>GVIKPDMKIKLKMEGNVNGHAFVIEGEGEGKPYDGTNTINLEVKEGAPLPFSYDILTNAFAYGNRAFTKYPDDIPNYFKQSFPEGYSWERTMTFEDKGIVKVKSDISMEEDSFIYEIHLKGENFPPNGPVMQKKTLKWEPSTEILYVRDGVLVGDIKHKLLLEGGG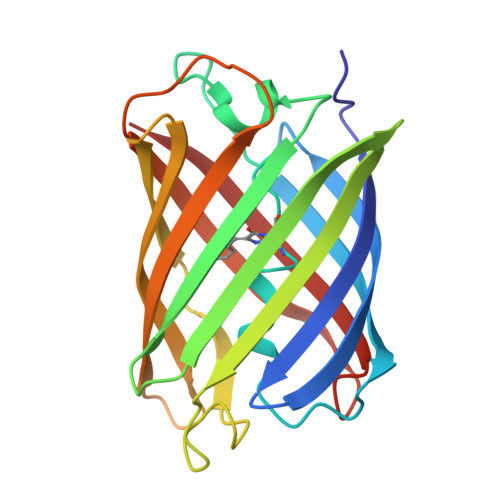HHRVDFKTIYRAKKAVKLPDYHFVDHRIEILNHDKDYNKVTVYESAVARY[2x]> MIIPALDLIGGTVVRVMRLHQGDYAR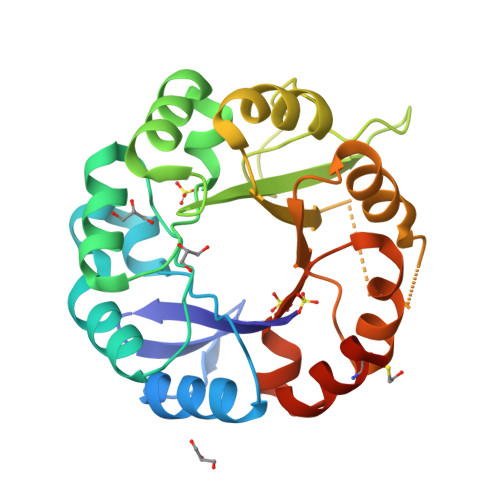LRDYGNDPLPRLQDYAAQGAGVLHLVDLTGAKDPAKRQIPLIKTLVAGVNVPVQVGGGVRTEEDVAALLKAGVARVVIASTAVKSPDVVKGWFERFGAQALVLALDVRIDEHGTKQVAVSGWQENSGVSLEQLVETYLPVGLKHVLCTDISRDGTLAGSNVSLYEEVCARYPQIAFQSSGGIGDIDDIAALRGTGVRGVIVGRALLEGKFTVKEAIQCWQNVKGHHHHHH>NEPAIEAFLQDGGTLAMLNDVSTDTLEQLYTLGFNQYHAGKHDEAHKIFQALCVLDHYEARFFLGLGACRQALGQFRLAIDSYSYGAMMDLQEPRFPFHAAECLLQLGELEGAESGFHSAQLLAAAKPELAELAARAGIMLEVVKTKKDME[4x];>[4x]GQGVVLPQPMPGIGQQMSPPKQQELDQLRKTAQLGTANAAKLLGSSTLLNKLAFASPEEFEIELSKMTSEL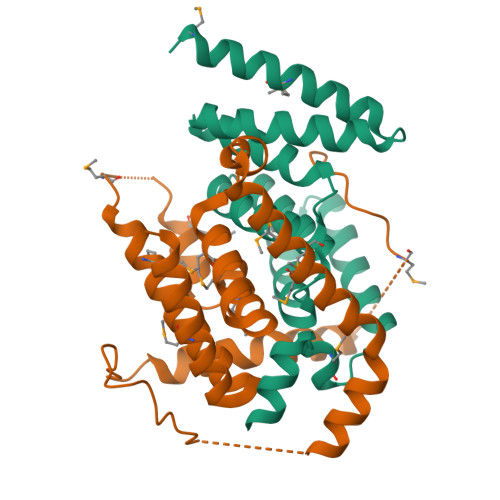EQTQKKLKLADLERIRAENLKKIDENQTKMKEASEAADKAKKSGLASKIFGWISAIASMVIGAILIATGVGAAVGAMMIVGGAVGVANMAIQQAAADGRISPETMKVLGPIMIAAEILVAIVSIAVTFGASAASTAMKAVKFATQAAD> MKPFLLGLLKCKRCSFMTKLILECEKAESNDVDTDDVK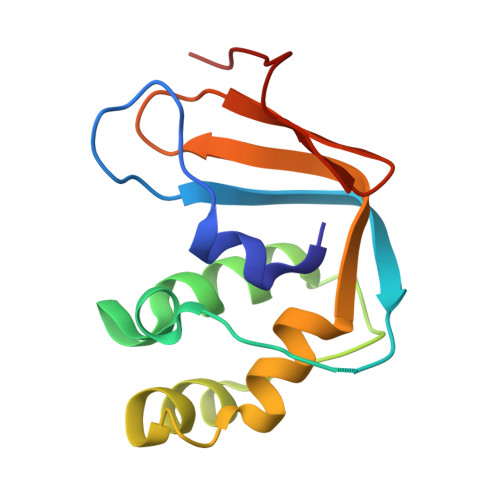IFNKHMFTENGGERLKSLVNSLRDFHGRELSEQDISSFVENPGDDEKIKEFLFGIDVVEGSLRCDMCGLIYPIKGSIVETVDTVESK>PGAPWWKSAVFYQVYPRSFKDTNGDGIGDFKGLTEKLDYLKGLGIDAIWINP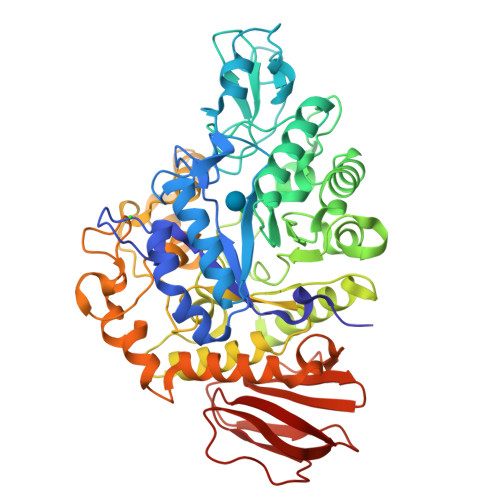HYASPNTDNGYDISDYREVMKEYGTMEDFDRLMAELKKRGMRLMVDVVINHSSDQHEWFKSSRASKDNPYRDYYFWRDGKDGHEPNNYPSFFGGSAWEKDPVTGQYYLHYFGRQQPDLNWDTPKLREELYAMLRFWLDKGVSGMRFDTVATYSKTPGFPDLTPEQMKNFAEAYTQGPNLHRYLQEMHEKVFDHYDAVTAGQIFGAPLNQVPLFIDSRRKELDMAFTFDLIRYDRALDRWHTIPRTLADFRQTIDKVDAIAGEYGWNTFFLGNHDNPRAVSHFGDDRPQWREASAKALATVTLTQRGTPFIFQGDELGMTNYPFKTLQDFDDIEVKGFFQDYVETGKATAEELLTNVALTSRDNARTPFQWDDSANAGFTTGKPWLKVNPNYTEINAAREIGDPKSVYSFYRNLISIRHETPALSTGSYRDIDPSNADVYAYTRSQDGETYLVVVNFKAEPRSFTLPDGMHIAETLIESSSPAAPAAGAASLELQPWQSGIYKVK[2x]> DPMAAERKTRLSKNLLRMKFMQRGLD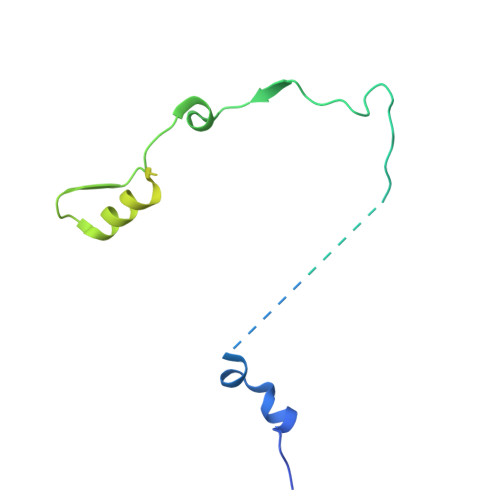SETKKQLEEEEKKIISEEHWYLDLPELKEKESFIIEEQSFLLCEDLLYGRMSFRGFNPEVEKLMLQMNAKHKAEEVEDETVELDVSDEEMARRYETLVGTIGKKFARKRDHANYEEDENGDITPIKAKKMFLKPQD> ITKSSKSSFSVLDIGLPMSALQRKMMHRLVQYFAFCIDHFCTGPSDSRIQEKIRLFIQSAHNIAKHPSLYDTEVRNPSAAESTNSHVSLDASNFSSYAENSSKFLFLQELFKNLSPSYSKTFFLFISNQFLANTLTQWLKSQNIDAELWAEEDAKTS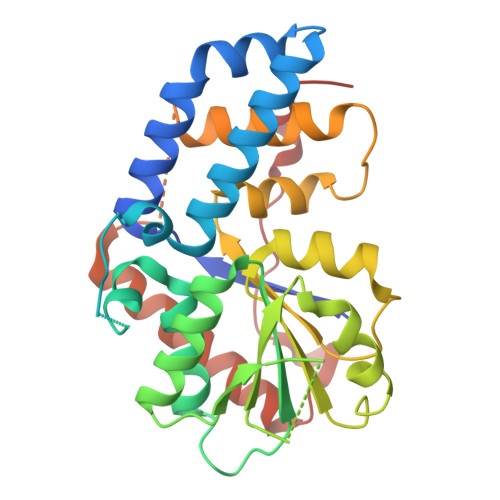QHPAIWICVSKKAPSASHFLQSCPDLSATIFYDIEAYMSVTSSLPSIQSLVLRLIHLGSIEHAIKCFQSSYNASFLVNIVGVVATLSSSSEENSEASNLSTLFEKSGNFEEILGSESHSSITEKTRDIAKNVATWLKNGENFSSWPLPPLMDLASLSVAE>MEQQPLTLTAATTRAQELRKQLNQYSHEYYVKDQPSVEDYVYDRLYKELVDIETEFPDLITPDSPTQRVGGKVLSGFEKAPHDIPMYSLNDGFSKEDIFAFDERVRKAIGKPVAYCCELKIDGLAISLRYENGVFVRGATRGDGTVGENITENLRTVRSVPMRLTEPISVEVRGECYMPKQSFVALNEEREENGQDIFANPRNAAAGSLRQLDTKIVAKRNLNTFLYTVADFGPMKAKTQFEALEELSAIGFRTNPERQLCQSIDEVWAYIEEYHEKRSTLPYEIDGIVIKVNEFALQDELGFTVKAPRWAIAYKFPPE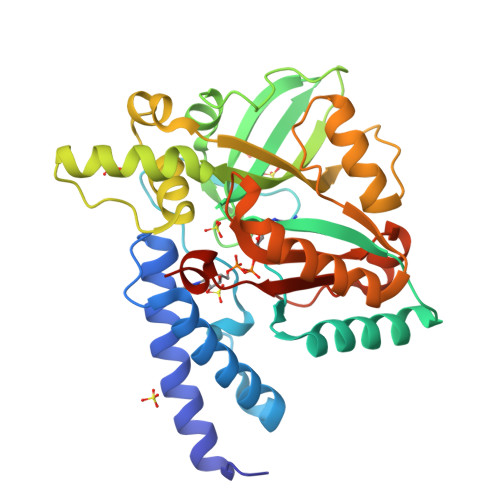EAETVLEHHHHHH[4x]>[2x]MGSSHHHHHHSQDPMTVTANQVLRPRGPQIERLTDNRAKVVIEPLERGYGHTLGNALRRVLLSSIPGFAITEVEIDGVLHEYTTVEGLQEDVLDVLLNLKDVAIRMHSGDSATLSLSKQGPGTVTAADIRTDHNVEIINGDHVICHLTKDTALNMRLKIERGFGYQPAAARRRPDEETRTIGRLMLDASFSPVRRVAYAVEAARVEQRTDLDKLVIDIETNGTIDAEEAVRTAADILSDQLSVFGDFTHRDRGAAKPAASGVDPVLLRPIDDLELTVRSANCLKAESIYYIGDLIQKTEVELLKTPNLGKKSLTEIKEVLAQRGLALGMKLENWPPAGVAQHGMLG;> MTSYSFTEKKRIRKDFGKQRSILEVPFLLAIQVDSYREFLQEDVESTKRKDLGLHAALKSVFPISSYSGNAALEYVGYKLGQPVFDERECRQRGMSYGAPLRVTVRLVIYDRESSTKAIKYVKEQEVYLGEIPLMTGNGTFIVNGTERVIVSQLHRSPGVFFDHDRGKTHSSGKLLYSARIIPYRGSWLDFEFDPKDALFTRIDRRRKLPVSILLRALGYNNEEMLAEFFEINTFHINPDEGVQLELVPERLRGETLNFDLADGDKVIVEAGKRITARHVKQLEAAGVAALAVPDDYLVGRILSHDVVDGSTGELLANANDEISEDQLTAFRKAGVDAVGTLWVNDLDRGPYLSNTLRIDPTKTQLEALVEIYRMMRPGEPPTKEAAQNLFHNLFFTFERYDLSTVGRMKFNRRVGRKDVLGESVLYDKKYFAERNDEESKRLVAEHTDTSDILEVIKVLTEIRNGRGVVDDIDHLGNRRVRSVGEMAENVFRVGLVRVERAVKERLSMAESEGLTPQELINAKPVAAAIKEFFGSSQLSQFMDQNNPLSEVTHKRRVSALGPGGLTRERAGFEVRDVHPTHYGRVCTIETPEGPNIGLINSLAVFARTNQYGFLETPYRKVLDGKVSDDVEYLSAIEENEYVIAQANALTDAKNMLTEQFVPCRFQGESLLKPPSEVHFMDVSPMQTVSVAAALVPFLEHDDANRALMGANMQRQAVPTLRSQKPLVGTGIERAVARDSGVTVNALRGGVIEQIDAARIVVKVNEAEIGGGTDAGVDIYNLIKYTRSNQNTCINQRPLVNVGDVIARGDVLADGPSTDIGELALGQNMLIAFMPWNGYNFEDSILLSERVVEEDRYTTIHIEELTCVARDTKLGPEEISADIPNVSEQALNRLDESGVVYIGAEVRAGDIMVGKVTPKGESQLTPEEKLLRAIFGEKASDVKDSSLRVPPGMDGTVIDVQVFTRDGIEKDKRARQIEENEIKRVKKDFDDQFRILEAAIYARLRSQIVGKVANGGANLKKGDSVTDAYLDGLKKSDWFQLRMKDEDAADAIERAQKQIQAHEKEFEARFADKRGKITQGDDLAPGVLKMVKVFLAVKRRIQPGDKMAGRHGNKGVVSNVVPVEDMPYMATGESVDIVLNPLGVPSRMNIGQILEVHLGWAAKGLGRKIQRMLEAQAAVSELRKFLDDIYNHDNAINAQRVDLSQFSDEELLNLGKNLIDGVPMATPVFDGASEAEIKRMLELADLPQSGQTQLYDGRTGEAFDRKTTVGYMHYLKLNHLVDDKMHARSTGPYSLVTQQPLGGKAQFGGQRFGEMEVWALEAYGAAYTLQEMLTVKSDDVQGRNQMYKNIVDGEHEMVAGMPESFNVLVKEIRSLAIHMELEE;> MKDLLNLFNQQRQTLDFDAIKIALASPDLIRSWSYGEVKKPETINYRTFKPERDGLFCAAIFGPIKDYECLCGKYKRMKHRGVVCEKCGTEVTLAKVRRERMGHIDLASPVAHIWFLKSLPSRIGLMLDMTLRDIERVLYFEAYVVTEPGLTPLERRQLLTEEQYLTARQEYNDDFDAAMGAEAVYELLRTIDLQSEMTRLREEIASTGSETKLKRLTKRIKLIEAFLESGNRPEWMVMTVLPVLPPDLRPLVPLDGGRFATSDLNDLYRRVINRNNRLRRLLELNAPDIIVRNEKRMLQESVDALLDNGRRGRAITGTNKRPLKSLADMIKGKQGRFRQNLLGKRVDYSGRSVITVGPYLKLHQCGLPKKMALELFKPFVFAKLQRRGLATTIKAAKKLVEREEAEVWDILEEVIREHPVLLNRAPTLHRLGIQAFEPVLIEGKAIQLHPLVCTAFNADFDGDQMAVHVPLSLEAQLEARALMMSTNNILSPANGEPIIVPSQDVVLGLYYMSRALENKKGEGMVFANTSEVKRAYDNRVVELHAKVKVRITQVDVDAVDGKRTSGTSIVDTTVGRALLSEILPEGLPFQLANTEMTKKNISRLINSSYRLLGLKDTVVFADKLMYTGYAYATRAGVSIGIDDMLIPDEKKGILTEAEAEVLEIQEQYQSGLVTAGERYNKVVDIWSRTSERIAKAMMDTIGTEKVENAKGETIDQKSMNSLYIMADSGARGSQAQIRQLAGMRGLMARPDGSIIETPIKANFREGLNVQEYFNSTHGARKGLADTALKTANSGYLTRRLVDVAQDVVITEIDCGTTEGLIMTPIVEGGDVVEPLKERVLGRVVAEDVYLPGNDEEPIVTRNTLLDEAWVAKLEDASVQSVKVRSTISCESSFGVCARCYGRDLARGHQVNIGEAVGVIAAQSIGEPGTQLTMRTFHIGGAASRAAAVDNITVKTTGSVKFNNLKSVAHASGSLVAVSRSGELSVLDGHGRERERYKLPYGATITAKDGDAVKAGQSVANWDPHNHPIVSEVAGFIRFIDFVDGVTVIEKTDELTGLASREITDPKRRGAHAKELRPIVRIVDGKGNDLTIPNTDLPAQYLLPPRSIVNLQDGAAVGVGDVVAKIPQEASKTRDITGGLPRVADLFEARKPKDPAILAERSGIISFGKDTKGKQRLIIKDTDGSEHEELIPKYRQIIVFEGEHVTKGETVVDGEPSPQDILRLLGVEPLAAYLVKEIQDVYRLQGVKINDKHIEVITRQMLRKVEIVDQGNSKFLNGEQVERQRVIEENARLVKRNELPAKYDPVLLGITKASLATESFISAASFQETTRVLTEAAVRGTRDNLRGLKENVIVGRLIPAGTGLAYHAGRRKASGLTDSEMETLSGKPAGAEPVAALADAGADEE;> MARITVEDCLEVVNNRFELVMMASKRARQLANGVQPLIENAAASDKPTVMALREIAARRIDNALIDEVEKAERERAEREALEWAAAEVVADEDMSKNDD;> GAMDMSKELLLVVDAVANEKGVPREVIFDAIEAALASAAKKRYPDQDVLARVTIDHKDGTYETYRRWEVVADDVVMESPDRQVRLMDAIDEADGVDVGDYIEEQIENPDFGRIAAQAAKQVIVQRVREAERQQVVDAWKDRVGELITGVVKRAERGNIFVDLGGNAEAFIPKDKGIPRDVLRPGDRVRGYLAEVRSEPRGPQLFISRAAPEFMIELFKLEVPEVGQGLVEINACARDPGDRAKIAVIAHDARTDPIGACIGMRGSRVQAVSNELNGERVDIVLWNENPANFVINAMAPAEVQSIIVDEDKHSMDLAVAEDRLAQAIGKGGQNVRLASRLTGWQLNVMTADQVAAKSEAEQAAARQLFMDRLEVDEEISAILVSEGFNTVEEIAYVPVGELLAVEGFDEDIVEELRARARDALLNAALAEEEGLEGTQPTEDLLALEGMDEETAVALAEHGVRTSEDLSDLAADEIVDFGIEGLTQERAAALILAARAEEIARLERGE;> GAMAMNEFTQISGYVNAFGSQRGSVLTVKVENDEGWTLVEEDFDRADYGSDPEFVAEVSSYLKRNGGIKDLTKVLTR

P7 is the key phage protein to regulate gene expression programs of both host bacteria and phage Xp10. P7 binds to host RNA polymerase to inhibit transcription of host genes. P7 turns on transcription of late genes of phage Xp10 by assisting host RNA polymerase in bypassing intrinsic terminators preceding the late genes. The structures reveal a unique binding site (the RNA-exit channel) of the phage protein P7 on bacterial host RNAP, where P7 exerts dual regulatory activities on host RNAP—inhibiting transcription initiation and preventing transcription termination.

The cryo-EM map of P7-NusA-TEC shows clear electron densities for 6-bp upstream double-stranded DNA (dsDNA), 9-bp DNA-RNA hybrid of the transcription bubble, 3-nt single-strand RNA (ssRNA) in the RNA exit channel, and 13-bp downstream dsDNA. The RNAP clamp in the P7-NusA-TEC is closed and the overall conformation of Xoo RNAP is essentially superimposable to E. coli TEC. The DNA–RNA hybrid in the P7-NusA-TEC adopts a canonical post-translocation conformation as in E. coli TEC, suggesting that P7 does not affect the conformation of the DNA and RNA during processive transcription elongation. P7 inserts into the RNA exit channel and makes extensive interactions with RNAP with calculated interface of 1182 Å2. The C-terminal helix of P7 (residues 48–62) forms a four-helix bundle with βCTR and β′dock. In the structure, NusA locates at outside of RNA exit channel, where it interacts with the tip helix of βflap domain (βFTH) with a hydrophobic groove of its NTD domain. P7 resides between NusA and the RNA exit channel of RNAP; the β2/β3 loop of P7 inserts into a cavity of NusA S1 domain and creates a moderate interface of 221 Å2. Specifically, the W32 of p7 inserts into a phenylalanine cage of F155, F165, and F200 on NusA. Structure superimposition between the Xoo P7-NusA-TEC and E. coli NusA-PEC reveals that the hairpin-interacting regions of NusA has been occupied by P7, explaining that NusA losses its activity of enhancing pause or intrinsic termination in the presence of P725.>ATCYCRTGRC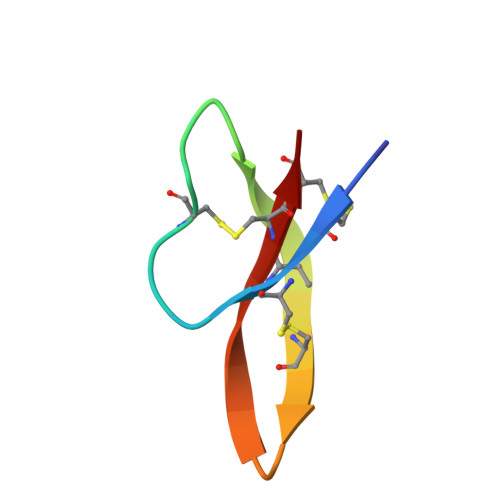ATRESLSGVCEISGRLYRACCR[9x]> SHMMGPKSKVFVPLYVYPAPGAWDPLEDVISKHPDVNFTVVINPGSGPGPEALPDGNYTREIPKLASYENVRLLGYVATTYAKRNIS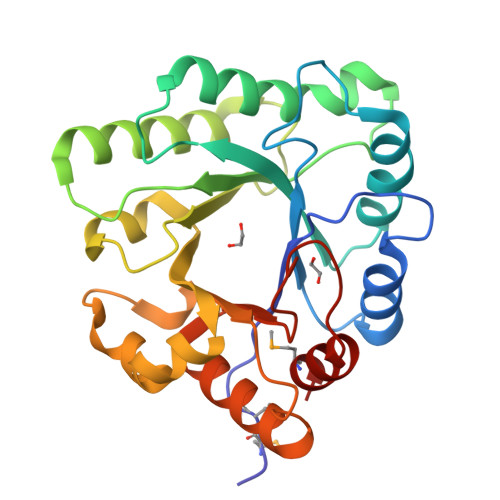EVRRDIETYAAWPTQSSNANLAVRGIFFDETPQQYDADILAYLRELTDVVKGTSGLGPDHYVVHNPGAIPDSRYLSTADSTVVFEATYATFQERHGAELFDTIPDSHRDQLCAVIHSVPTSVEGSDLRGLVKQVRQVADEIFITHLETDYYAGFGGQWSEFVDLMAS> AFARDPTQFEERHLKFLQQLGKGNFGSVEMCRYDPLQDNTGEVVAVKKLQHSTEEHLRDFEREIEILKSLQHDNIVKYKGVCYSAGRRNLKLIMEYLPYGSLRDYLQKHKERIDHIKLLQYTSQICKGMEYLGTKRYIHRDLATRNILVENENRVKIGDFGLTKVLPQDKEYYKVKEPGESPIFWYAPESLTESKFSVASDVWSFGVVLYELFTYIEKSKSPPAEFMRMIGNDKQGQMIVFHLIELLKNNGRLPRPDGCPDEIYMIMTECWNNNVNQRPSFRDLALRVDQI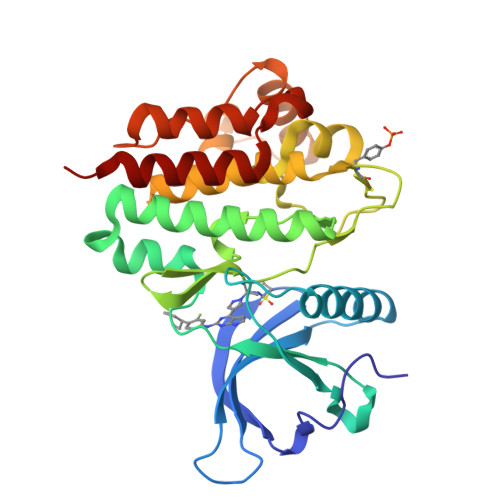RDNMAG>[2x]MAHHHHHHVGTGSNDDDDDKSPSKSSEKRQAVDTAVDGVFIRSLKVNCKVTSRFAHYVVTSQV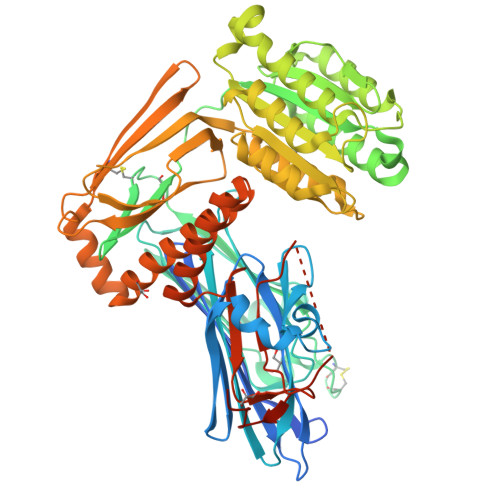VNTANEAREVAFDLEIPKTAFISDFAVTADGNAFIGDIKDKVTAWKQYRKAAISGENAGLVRASGRTMEQFTIHLTVNPQSKVTFQLTYEEVLKRNHMQYEIVIKVKPKQLVHHFEIDVDIFEPQGISKLDAQASFLPKELAAQTIKKSFSGKKGHVLFRPTVSQQQSCPTCSTSLLNGHFKVTYDVSRDKICDLLVANNHFAHFFAPQNLTNMNKNVVFVIAISGSMRGQKVKQTKEALLKILGDMQPGDYFDLVLFGTRVQSWKGSLVQASEANLQAAQDFVRGFSLDEATNLNGGLLRGIEILNQVQESLPELSNHASILIMLTDGDPTEGVTDRSQILKNVRNAIRGRFPLYNLGFGHNVDFNFLEVMSMENNGRAQRIYEDHDATQQLQGFYSQVAKPLLVDVDLQYPQDAVLALTQNHHKQYYEGSEIVVAGRIADNKQSSFKADVQAHGEGQEFSITCLVDEEEMKKLLRERGHMLENHVERLWAYLTIQELLAKRMKVDREERANLSSQALQMSLDYGFVTPLTSMSIRGMADQDGLKPTIDKPSEDSPPLEMLGPRRTFVLSALQPSPTHSSSNTQRLPDRVTGVDTD>[3x]GSHMAKVYIEEKPKVTFKDVAGIEEVKEEVKEIIEYLKDPVKFQKLGGRPPKGVLLYGEPGVGKTLLAKAIAGEAHVPFISVSGSDFVEMFVGVGAARVRDLFETAKKHAPCMIFIDEIDAVGRARGAIPVGGGHDEREQTLNQLLVEMDGFDTSDGIIVIAATNRPDILDPALLRPGRFDRQIFIPKPDVRGRYEILKVHARNKKL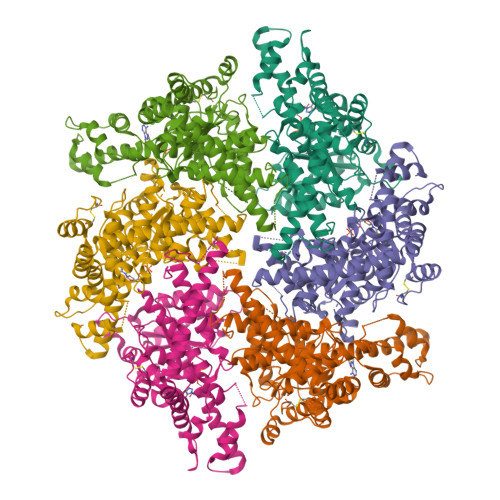AKDVDLEFVARATPGLTGADLENLLNEAALLAARKGKEEITMEEIEEALDRITMGLERKGMTISPKEKEKIAIHEAGHALMGLVSDDDDKVHKISIIPRGMALGVTQQLPIEDKHIYDKKDLYNKILVLLGGRAAEEVFFGKDGITTGAENDLQRATDLAYRMVSMWGMSDKVGPIAIRRVANPFLGGMTTAVDTSPDLLREIDEEVRRIITEQYEKAKAIVEEYKEPLKAVVKKLLEKETITCEEFVEVFKLYGIELKDKCKKEELFDKDRKSEENKELKSGEVKEEVV>MGCCSSASSAAQSSKREWKPLEDRSCTDIPWLLLFILFCIGMGFICGFSIATGAAARLVSGYDSYGNICGQKNTKLEAIPNSGMDHTQRKYVFFLDPCNLDLINRKIKSVALCVAACPRQELKTLSDVQKFAEINGSALCSYNLKPSEYTTSPKSSVLCPKLPVPASAPIPFFHRCAPVNISCYAKFAEALITFVSDNSVLHRLISGVMTSKEIILGLCLLSLVLSMILMVIIRYISRVLVWILTILVILGSLGGTGVLWWLYAKQRRSPKETVTPEQLQIAEDNLRALLIYAISATVFTVILFLIMLVMRKRVALTIALFHVAGKVFIHLPLLVFQPFWTFFALVLFWVYWIMTLLFLGTTGSPVQNEQGFVEFKISGPLQYMWWYHVVG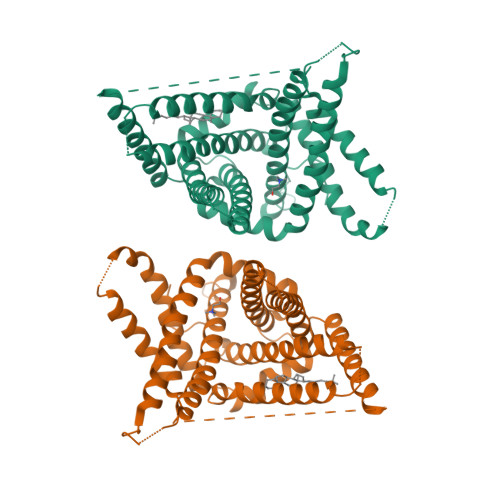LIWISEFILACQQMTVAGAVVTYYFTRDKRNLPFTPILASVNRLIRYHLGTVAKGSFIITLVKIPRMILMYIHSQLKGKENACARCVLKSCICCLWCLEKCLNYLNQNAYTATAINSTNFCTSAKDAFVILVENALRVATINTVGDFMLFLGKVLIVCSTGLAGIMLLNYQQDYTVWVLPLIIVCLFAFLVAHCFLSIYEMVVDVLFLCFAIDTKYNDGSPGREFYMDKVLMEFVENSRKAMKEAGKGGVADSRELKPMASGASSA[2x]quinoline-3-carbonitrile | C10 H6 N2 | 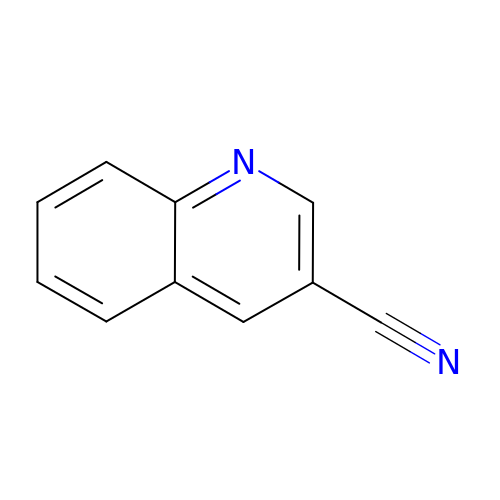QZZYYBQGTSGDPP-UHFFFAOYSA-N Altogether CD38 appears to be a key player in the biosynthesis of calcium messengers which are involved in a wide range of cellular functions. Thus, the catalytic transformation of NAD+ involves the formation, via a ribooxocarbenium ion-like transition state, of a unique reaction intermediate that partitions between several competing pathways such as an irreversible hydrolytic process leading to ADP-ribose and a reversible minor pathway that governs the formation of cADPR. The L-shaped structure of bCD38 consists of two distinct domains separated by a cleft and connected by a hinge region. α-Helices are found mainly in the N-terminal and membrane-proximal domain of this transmembrane protein, whereas β-sheets are preponderant in the distal C-terminal domain. The active site of bCD38 consists in a funnel-shaped cavity with a fairly rigid structure; it buries the NMN+ moiety of the substrate and its scissile bond in its deepest non-polar and least solvent accessible region, whereas the AMP moiety interacts with its more solvent-exposed region, at the entrance of the catalytic cleft.

Next we replaced NAD+ with 2′-deoxy-2′-β-D-fluororibofuranoside NAD+ (rFNAD), a close (bioisosteric) structural analog carrying a fluorine atom at position 2′ of the ribose moiety linked to nicotinamide (N-ribose). Using this strategy, we were able to trap a non-covalent complex between the E218Q mutant and rFNAD and its structure was solved at 1.94 Å. Despite the presence of two CD38 molecules in the asymmetric unit of E218Q mutant of bCD38, the structure of the non-covalent complex with rFNAD revealed that only one site is fully occupied; it is possible that one of the monomer and active site are rendered less accessible and/or reactive due to crystalline packing constraints. In particular the ribose from the adenosine part is well-resolved in density. This NAD+ analog is constrained by the enzyme in a somewhat folded conformation and is stabilized in the active site by extensive interactions. The electron density maps show that the nicotinamide ring of rFNAD is buried in the active site in agreement with the experimental observation that the cleavage of the nicotinamide-ribosyl bond is the first step of catalysis. Thus, the N7 atom of its carboxamide group is hydrogen bonded to Oε1 of the carboxylate group of Glu138 (d = 2.7 Å) and Asp147 (at a suboptimal distance = 3.3 Å). Upon formation of the Michaelis complex, this hydration network is disrupted and displaced by the binding of the N-ribose moiety of the ligand. As shown in Figure 4A in the rFNAD/E218Q complex the 2′-deoxy-2′-fluororibose linked to nicotinamide is fixed in the active site through efficient hydrogen bonds between its 3′-OH group, which displaces a bound water molecule, and the Oε1 atom of the mutant residue Gln218 (d = 2.7 Å) and backbone NH group of Trp118 (d = 2.9 Å).

>[2x]YKWHYSGLNRWHGAGSTADFQKIIQERCDTYTQTIRPGSRSRNCQAIRQAFMSAFISKDPCKATKEDYNSLINLAPPTVPCGQQVFWSKTKELAHEYAKRRRLMTLEDTLLGYLADGLRWCGEPGSSDLNIWSCPDWRKDCRTNYLSVFWEVLSERFAESACNTVRVVLNGSLENAFDSMSIFGRVQAPNLRPQVELEAWLVHDTGKPPSDSCSGSSIRKLKSILDGRNVKFRCMDNLSRDQFLQRS> GSPALDTGTTEEDRLKIDVIDWLVFDPAQRAEALKQGNAIMRKFLASKKHEAAKEVFVKIPQDSIAEIYNQCEEQGMESPLPAEDDNAIREHLCIRAYLEAH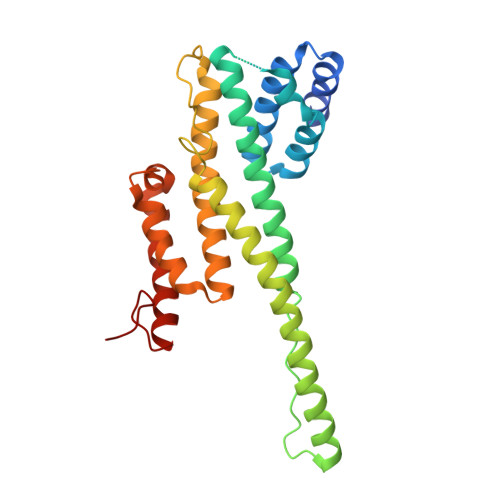ETFNEWFKHMNSVPQKPALIPQPTFTEKVAHEHKEKKYEMDFGIWKGHLDALTADVKEKMYNVLLFVDGGWMVDVREDAKEDHERTHQMVLLRKLCLPMLCFLLHTILHSTGQYQECLQLADMVSSERHKLYLVFSKEELRKLLQKLRESSLMLLDQGLDPLGYEIQL> RSSHHHHHHGEFDDPIRPPLKVARSPRPGQCQDVVQDVPNVDVQMLELYDRMSFKDIDGGVWKQGWNIKYDPLKYNAHHKLKVFVVPHSHNDPGWIQTFEEYYQHDTKHILSNALRHLHDNPEMKFIWAEISYFARFYHDLGENKKLQMKSIVKNGQLEFVTGGWVMPDEANSHWRNVLLQLTEGQTWLKQFMNVTPTASWAIDPFGHSPTMPYILQKSGFKNMLIQRTHYSVKKELAQQRQLEFLWRQIWDNKGDTALFTHMMPFYSYDIPHTCGPDPKVCCQFDFKRMGSFGLSCPWKVPPRTISDQNVAARSDLLVDQWKKKAELYRTNVLLIPLGDDFRFKQNTEWDVQRVNYERLFEHINSQAHFNVQAQFGTLQEYFDAVHQAERAGQAEFPTLSGDFFTYADRSDNYWSGYYTSRPYHKRMDRVLMHYVRAAEMLSAWHSWDGMARIEERLEQARRELSLFQHHDGITGTAKTHVVVDYEQRMQEALKACQMVMQQSVYRLLTKPSIYSPDFSFSYFTLDDSRWPGSGVEDSRTTIILGEDILPSKHVVMHNTLPHWREQLVDFYVSSPFVSVTDLANNPVEAQVSPVWSWHHDTLTKTIHPQGSTTKYRIIFKARVPPMGLATYVLTISDSKPEHTSYASNLLLRKNPTSLPLGQYPEDVKFGDPREISLRVGNGPTLAFSEQGLLKSIQLTQDSPHVPVHFKFLKYGVRSHGDRSGAYLFLPNGPASPVELGQPVVLVTKGKLESSVSVGLPSVVHQTIMRGGAPEIRNLVDIGSLDNTEIVMRLETHIDSGDIFYTDLNGLQFIKRRRLDKLPLQANYYPIPSGMFIEDANTRLTLLTGQPLGGSSLASGELEIMQDRRLASDDERGLGQGVLDNKPVLHIYRLVLEKVNNCVRPSKLHPAGYLTSAAHKASQSLLDPLDKFIFAENEWIGAQGQFGGDHPSAREDLDVSVMRRLTKSSAKTQRVGYVLHR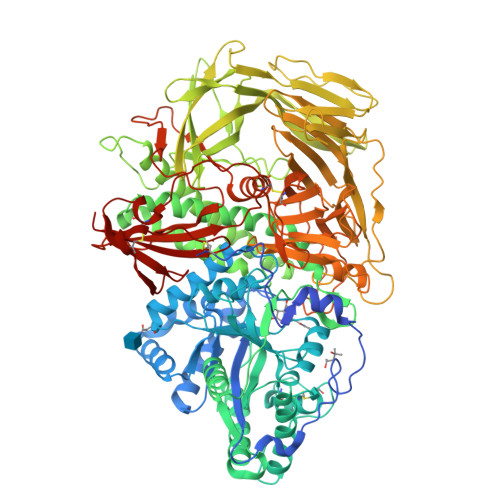TNLMQCGTPEEHTQKLDVCHLLPNVARCERTTLTFLQNLEHLDGMVAPEVCPMETAAYVSSHSS>MGFKEYPAGEPVTMNEMELAAVYLQPIDMEPRGMGLPAAKADVHLQADIHAVEGNKNGFGAGEWIPYLTISY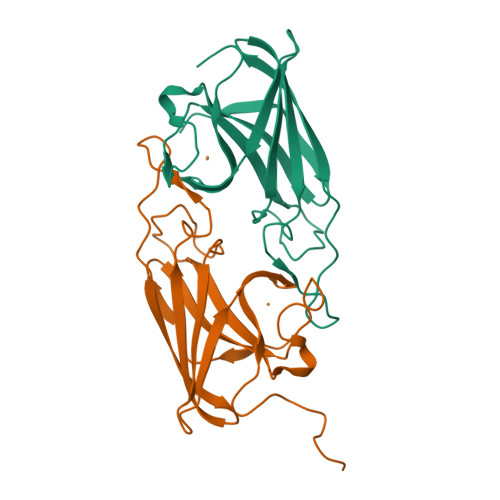TLVNNDTGEKQEGTFMPMVASDGPHYGANIKMMGVGNYKVTYHIEPPSKAGMHRHTDSETGVGRWWKPFDVSYEFKYVGLNSSGLVPR[2x]> MSTQYETQGYTINNAGRRLVVDPITRIEGHMRCEVNINDQNVITNAVSCGTMFRGLEIILQGRDPRDAWAFVERICGVCTGVHALASVYAIEDAIGIKVPDNANIIRNIMLATLWCHDHLVHFYQLAGMDWIDVLDALKADPRKTSELAQSLSSWPKSSPGYFFDVQNRLKKFVEGGQLGIFRNGYWGHPQYKLPPEANLMGFAHYLEALDFQREIVKIHAVFGGKNPHPNWIVGGMPCAINIDESGAVGAVNMERLNLVQSIITRTADFINNVMIPDALAIGQFNKPWSEIGTGLSDKCVLSYGAFPDIANDFGEKSL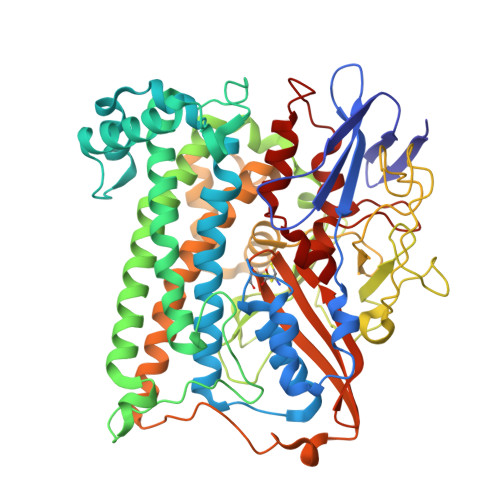LMPGGAVINGDFNNVLPVDLVDPQQVQEFVDHAWYRYPNDQVGRHPFDGITDPWYNPGDVKGSDTNIQQLNEQERYSWIKAPRWRGNAMEVGPLARTLIAYHKGDAATVESVDRMMSALNLPLSGIQSTLGRILCRAHEAQWAAGKLQYFFDKLMTNLKNGNLATASTEKWEPATWPTECRGVGFTEAARGALGHWAAIRDGKIDLYQCVVPTTWNASPRDPKGQIGAYEAALMNTKMAIPEQPLEILRTLHSFDPCLACSTH>[4x]NGLSNIVLTCKDLPIPIDLLSLFFDILNERHPSFD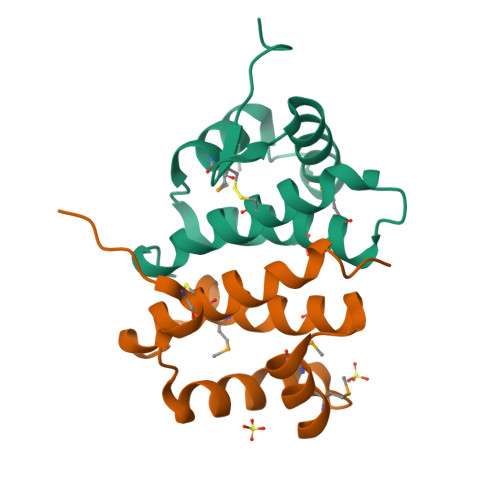EHMFLQMIRKPDDPENLSVFLKSAIWMLSHKRDLPGHYRLPLTCLVSTYSEYFVELKPR>[4x]MLNSFKLSLQYILPKLWLT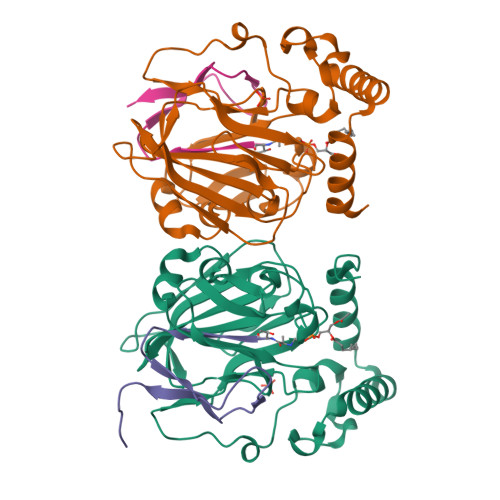RLAGWGASKRAGWLTKLVIDLFVKYYKVDMKEAQKPDTASYRTFNEFFVRPLRDEVRPIDTDPNVLVMPADGVISQLGKIEEDKILQAKGHNYSLEALLAGNYLMADLFRNGTFVTTYLSPRDYHRVHMPCNGILREMIYVPGDLFSVNHLTAQNVPNLFARNERVICLFDTEFGPMAQILVGATIVGSIETVWAGTITPPREGIIKRWTWPAGENDGSVALLKGQEMGRFKLG;>XTVINLFAPGKVNLVEQLESLSVTKIGQPLAVSTGHHHHHHG[4x]>[2x]MVIKAQSPAGFAEEY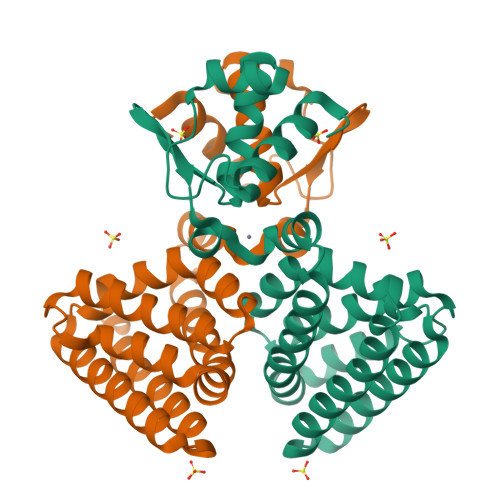IIESIWNNRFPPGTILPAERELSELIGVTRTTLREVLQRLARDGWLTIQHGKPTKVNNFWETSGLNILETLARLDHESVPQLIDNLLSVRTNISTIFIRTAFRQHPDKAQEVLATANEVADHADAFAELDYNIFRGLAFASGNPIYGLILNGMKGLYTRIGRHYFANPEARSLALGFYHKLSALCSEGAHDQVYETVRRYGHESGEIWHRMQKNLPGDLAIQGR>[3x]AGHMVSCCYRSLAAPDLTLRDLLDIVETSQAHNARAQLTGALFYSQGVFFQWLEGRP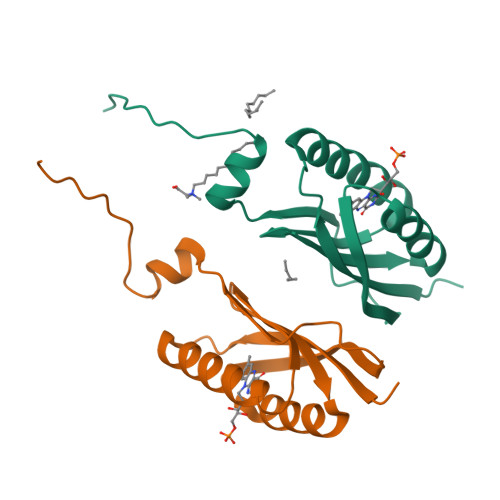AAVAEVMTHIQRDRRHSNVEILAEEPIAKRRFAGWHMQLSCSEADMRSLGLAESRQIVTVGRSL3-(3,4-dihydroxy-5-nitrobenzylidene)pentane-2,4-dione | C12 H11 N O6 | 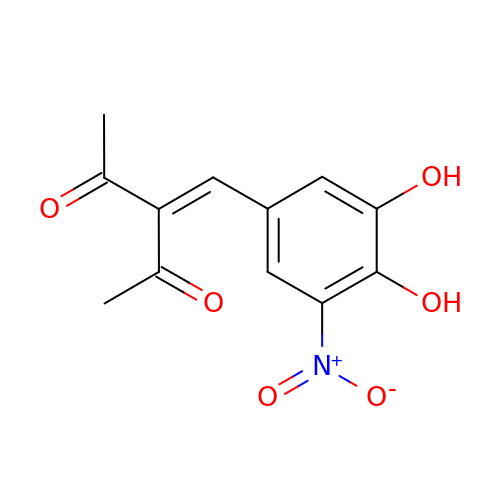UPMRZALMHVUCIN-UHFFFAOYSA-N> GADYDLKFGMVAGPSSNEYKAVEFFAKEVKEKSNGKIDVAIFPSSQLGDDRVMIKQLKDGALDFTLGESARFQIYFPEAEVFALPYMIPNFETSKKALLDTKFGQGLLKKIDKELNVQVLSVAYNGTRQTTSNRAINSIEDMKGLKLRVPNAATNLAYAKYVGAAPTPMAFSEVYLALQTNSVDGQENPLPTIQAQKFYEVQKYLALTNHILNDQLYLIS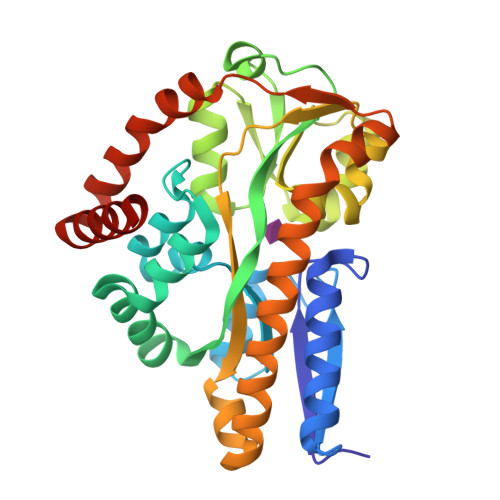NDTLADLPEDLQKVVKDAAAKAAEYHTKLFVDGENSLVEFFKSQGVTVTQPDLKPFKAALTPYYDEYLKKNGEVGKMAIEEISNLAKL>[6x]MIEMKPHPWFFGKIPRAKAEEMLSKQRHDGAFLIRESESAPGDFSLSVKFGNDVQHFKVLRDGAGKYFLW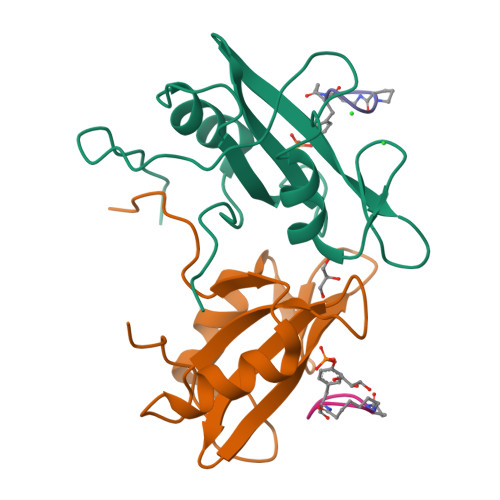VVKFNSLNELVDYHRSTSVSRNQQIFLRDIEQVPQQPTYVQA;>YVNVPX[6x]> MSKELTAKKRAALNRLKTVRGHLDGIVRMLESDAYCVDVMKQISAVQSSLERANRVMLHNHLETCFSTAVLDGHG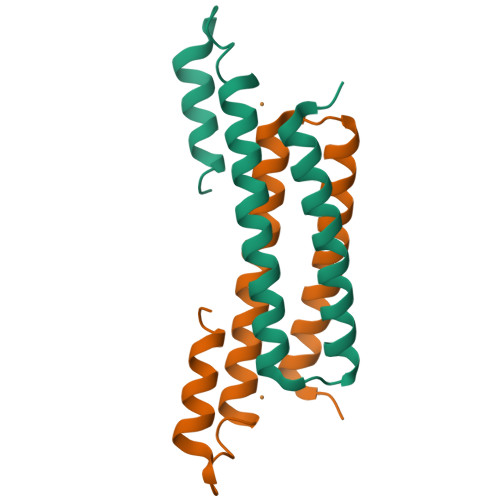QAAIEELIDAVKFTPALTGPHARLGGAAVGESATEEPMPDASNM> GEIEFIESSKDAGFPVINTPSKTKLEPSVFHQVFEGNKEPAVLRSGDPRLKANFEEAIFSKYIGNVNTHVDEYMLEAVDHYAGQLATLDISTEPMKLEDAVYGTEGLEALDLTTSAGYPYVALGIKKRDILSKKTKDLTKLKECMDKYGLNLPMVTYVKDELRSIEKVAKGKSRLIEASSLNDSVAMRQTFGNLYKTFHLNP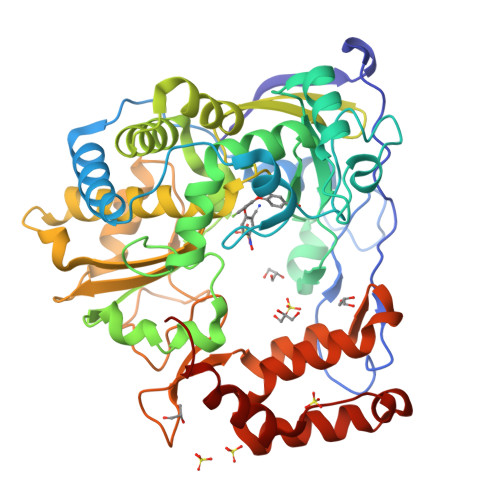GVVTGSAVGCDPDLFWSKIPVMLDGHLIAFDYSGYDASLSPVWFACLKMILEKLGYTHKETNYIDYLCNSHHLYRDKHYFVRGGMPSGCSGTSIFNSMINNIIIRTLMLKVYKGIDLDQFRMIAYGDDVIASYPWPIDASLLAEAGKGYGLIMTPADKGECFNEVTWTNVTFLKRYFRADEQYPFLVHPVMPMKDIHESIRWTKDPKNTQDHVRSLCLLAWHNGEHEYEEFIRKIRSVPVGRCLTLPAFSTLRRKWLDSFHHHHH>MALKDDAVLIAARGYVYTAAVGTAAPTPSQLKLIDLEHPEAWDRTGWDLVGHTSEDDLPEFGFDGGDSEVRGSWQKKKLREVETEEIADYVVINLTQFDETALELYFGPNQSATPGIFGVKSGSVVNERALLIVIVDNDVRLGFHARKASLKREDAISLATDEFGALPVRATFLDYQSYNLYEWIEEDWFNAVDAPVVYLLDLGGATGGDYTLLVGGKSTGDIAYNANASAIKTAIGAVDDGVAESAWTVTADGSDFEISGPLAVALGVDSTTGGSGVTVDVV[6x];>[3x]MTTVTATVHDISGRPDDSHWTFSSDLREQDGVIITPRVVRVKPFNGELALTLPPGPVRVTHHQDRWLIDVPEEDSDLWDLIEAATD;>MTVTITADVRDVTGQPDNQQWVFSTVLRQQDGSILTQKQVRVNPVDGALSVELEPGFAIVVYGEYRWFIEVPETDAGLWGLIATSVAVPPDTSAELLADAVNGYLDANPPSADWDALSNVPSEFPPSAHDHVAADVTDLDSAIAAYLASNPPEAGSVAWDDIDDKPSTFTPSSHTHSIANVTGLQDALDEKLDEAAVDARVSLGTAALVDSAPSTLDTLNELAAALGDDPNFATTVASQIGAKADKATTITAGTGLTGGGDLSANRTLNVSFGTSSTTACVGNDSRLSNTRTP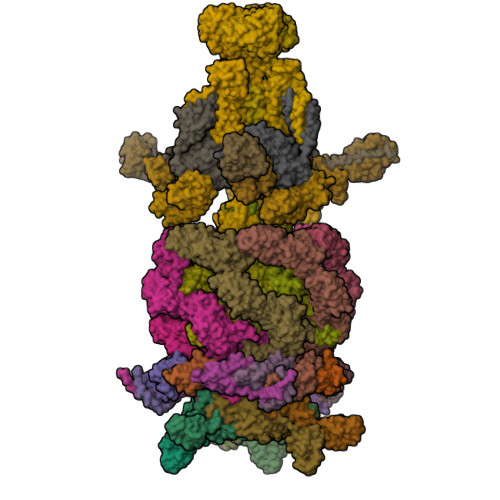TDGSVTNAKVASGAGIALSKLATGYVAGSDNSGARTLTIWVGTEAQYTAIGTKDSNTIYLRTA[9x];>[6x]MASRLLDPDTLVELEGVNGEWFDLTNGTEGIYLATEVTGLLDPPVKATYEEPGNFPGARYLNHRVLRRDLVFGVEILNDENDETWLRRDSAWRKAWSFKRDAKLHITTGESGHRYLKVRLFESPTTDMVTDPRGREVNITKMVVVAGDPFWYEDDVVYPIEVQEDTTFDPNPLPWPWPQPELPVEDIEITVPNANPTDNIIWPKWTLPGSSEKPAEPYIPGLPWLGAPKSPATLWTVPDYKLDLDEDEDPSLGTRRIRMPGQIGGLRVEEVQQIYIDGRPTGGTFKIGYGDEWTEPIAYNASPNDVRAALIALEGISANDVEVSLGGATNEVQTVRLKGGALGGTFTLSLGSETTVGIPFNASDADLQGALVGLDSIGSADVRVKSTKINEVQVVELVGEPTSGSFTLTLDGQTTAPIAYNATPATVAARIADLPNIDGNYVKVEGLNEWFHSPYRITFGEAQSQGVITDIISGIIDFIGGLFGGNASGKGVGGIDIDEMTGDVGTLSGGAGLDVQVTTEQDGDRLYVVSFQRAAGGLNLPQLVGNASGLEGDDLSIETATNVDGGRPYVVRFTDDLQGVDVPTMTVDTDDLTGGYEVGSRVVVLREGYTYPAENVVVDSDPREEQVSSESGSPIWERMNSVRFLHYIPPYTGEVTFKLSVSGAVPGQIATLRLPRAWSRPWGLE;>MAAGKEVGRLSIKVTPDLDGFYRELKAAVEAAEKMKVHIPVEPDMGNFRQEVAASTAGMSTRVKVQADVDRGLLDRLSNSLSGMKAPSFGSGINPTGYMLILGAAAALTPLIAGSLGAISAALLTLPGLIAAVAVPIGALALGIDGFKRAAERLKPAFDGLKESMSAAVENQFGPVFDQLGKAIPTLAANLPKVTQGMADVAKSIVDSVTSGEGLGRIESLISNIGAAISRSAPGLTSFVDGLLNLAEKFSGKLPAIADWINRTGESFSKWVTDFTTAGPDGVSKFDNAMSGLGDTLQMLGGGLVDILNKSLEFFSDPQKIQSFKAELDGLIASISTLVDLINSLAAAFSKVPGLSDGEANGVMDFAPIQIQGAIELIKQIPTAWEGVKLKAAEVWNSIPTMAATAIASIRATLATLPGLLSGIWTTVTASASSAFATIGAAVSAGARSVVNTAGNIFRSMGSVIANAFSAAVSAVQTAFSQMVSAAASGAQQVVAEVQALGGKIAAAAGNFGSILVAAGKALMDGLLSGIKAGLSAVLDFASGIAAKIAAVKGPLPKDRKELIPAGEALMEGLGTGIENGLDPVLDRAREIAKQIFSAFKETFGTAPTSLAFNLGSMQGDLSGLQTSLESTATASRDLTSSLTAPTAELASGSSLLGDDVKDQLDELKLAYDQLELQRKQLKVQKNEAGSKEDKAAIQDKIDALQAEKDKLAYQKDQLKIQQKQTGEMGEQKTLAQFLGEQIASTWQQGTDAVAGFARSNLDQAMSDLGIGGGAITNGLNAGLDWGVQALGNAVNIQVNSVDDAIAVKNNEVNKQALTYTRR[3x];>MPAPAADMTTLAGHQQLWDTVMKRRQKREDERIAPPLIRLWDGDYKLRGQLVGERSHKFEFIENETGTASITISLDHYLAKWIASHKGRARRNVHVSFDKQGARWTGRMDHYDIVRTKEGDVYMEVVFKHDYEELKHIYVWANPFLRPEFQFPKLWVMFGPAKWALLLTLFVNILRLETSLWTLPDNPLDISEWFPFSLNPGNWRNIVKPFPFLADNSPLTIVFSRFKSFHDTAKNVLADSQLTIVCRRYFHGEDPHPFAELSGELGLPLIEGIASLIPLRHGCLVWDIVDNSGWGSETAFGGSLLTGLVRAVMNIASDGMTEGIDIYTGLPTYPGEYYTPGFLGTYPKAPHVVFMESPYTGIESSKFTYTEATDTSFVLGGQSMPGVNEVISAGINMGGDFLTSLINSQLATLGAFGGAIDLPPLGGIMDAVARPLYENVVLAFMEIPTLRAAGLSLPIAGLEDIVTGLGDFHYNEGWVDGADKAFTISAIMAARAKQWATRAKHSHEIQVSDAAPYIIGERGHGHFWLGDRVGTTVLGYPDPYTIFVERVTKLTYEWTSDGPKGWTITIGYKEPEDPILKAFELIQYINSNLGQLGIL[3x];>MADDQWVPDVPDGAFVIGGGDYRYGQDMTEDIARSLFQVPDFNPANALLVLPQLLLRLPLEALQKFKDFIPNVLEGAFNTVAGAVDAIMGAIRETPRVLEQILSYLPQELRDELEHAAARIGAVIDAIVQALTGTLNIGHTIEDLIFSLTNIRPGAVGGVLGGGSIEETIKRIVDAIVSGIVGVTGIGAGISDLQSLIEQISSAAARGGFAWDILGIQNNKKPKSGLYKSERGNFDLDTLNSTVSVAPGTSIIAFDVIEQSMPIGLITWIGWGTSGITEFYINVYRCVDDRSDPELGELIHQSENIAGLLAGSASPGANMAYELTTPIEAVAGDLLAYEFIAVGGTHTMRGRDFNLPDNDGAPIGNVGATRSLSTPSLPPATLDKADVTWTDNVPRVGIAVDTGTGSDHHDPQVEFFEKPVAIPVPAWCDRIDAIVTGKGGEGADGFLGFYGNPGQPGSVNTVTWTRGEHFSGTTTILEWDGAELSIPGFEVSAANGSNGSGQRPVALGKPVGKGIEEVEYNGLKLAAGGDQHAYGGAGTKPGGGGNGGHWLGIYTQGGPGGPACAAVQFRKGALPGEVVGDGEGDVTPPNVSALHVDVSATSTSITITPSGAVDDA[3x];>[3x]MSLKVGGLDVVGVFVGDAAATIYVGAMRIWPPVPDFTPFTISSEDPGYEDLIDEQVPEGASGCWVTLGGAGGGGGSGRRANSGYRYGGGGGGGGGYIDRVWIPRASLGSTFTLIRGLGGAGGARAAGSSNGNNGAPGGSTVFSSGSVSLTASGGAAGVKGTSSSASGSGGAGGTTSISGVSATGYTGGKGGNGGSSPSSGQSRTDGSGAGGGGGGGVRSNDNSFSGGSNGTSSGPAGNGGRGTDGSINTGGSNAGSGGDGYVLIEWE;>MIDADDYTVNLTSHTTLANIPSGAIIAVSESLTGKSVTSAGWVKADPTVFPEVTGDTGEAVIVYKHTGTASTSTLLSYHDSPTYQFVIPNGSDIRVIWPTDGFIRF[6x];>MPSGLRGYNVYRNGVRQNTSPVTELGSVTITGLTPGTDYSSQITVTAIDMAGNESEPKTLAELEAEAATDELSPADPLAPAVRAQIDALVAAKMKPTSGKEADGAMVGIETPTGSYYKAYGGDRTKNQPLFLEQNFRYGSCSKMACNTLLLREIDRGHVDWDDTLDQFIDGIPNGDKITVRYLLLFQDGLKDWLQGDPAVQQTYFLNPTLNYDPLAYIRASTPVFEPGTDSHYSNAATLLMGKILEWCDAEFYTGRSARELIVEEWKNTVGMESLHWPTTNYMNQPYVRGWTPNMALPQIQAILGPFAFLAGLLGYPTSKDLEWTAVSTTWSDAAGSLAGNMEDFVKFGKALYEGEFLSEEMNQLRKEIFTRYVEYEPAGPHQGPGWMGFGLNSICWGHWLGWVGNLGGYIAVLFYNQDDGSVIATMLNNFAGHADAVDLFYQIAYLLNPESTGHRDWIFRPDPAEDADEVRDPTLYLTVESTGDNQIPADVPFEI[3x]1(R)-1-ACETAMIDO-2-(3-CARBOXY-2-HYDROXYPHENYL)ETHYL BORONIC ACID | C11 H14 B N O6 | 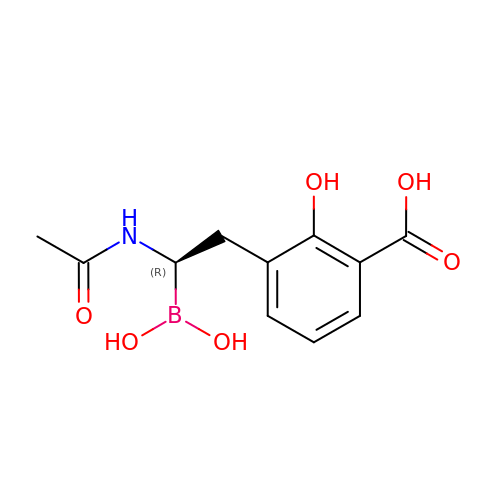MSRKDROGGGBNIX-VIFPVBQESA-N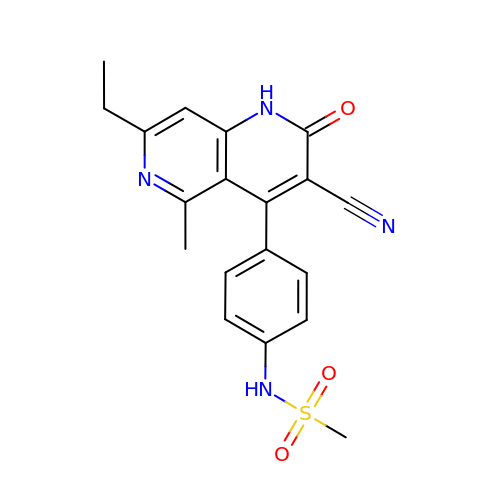N-[4-(3-CYANO-7-ETHYL-5-METHYL-2-OXO-1H-1,6-NAPHTHYRIDIN-4-YL)PHENYL]METHANESULFONAMIDE | C19 H18 N4 O3 S | RGARWRHBMWUMJL-UHFFFAOYSA-N>[2x]MPL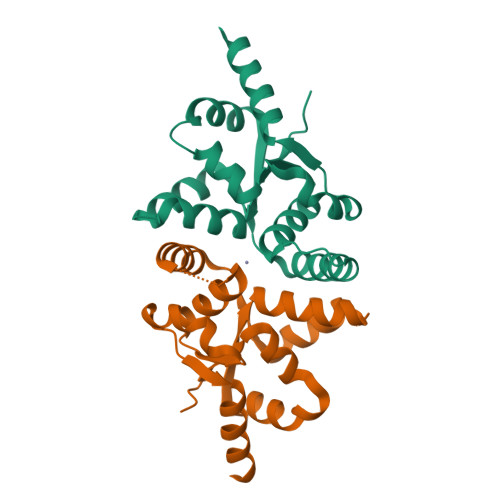PPDITFDSLALIKMHSQNMKRILEVTLAKFTVNLSIVTVYRYLTARAYLKKNIEAEFEILKDIYNIVPLLDDIAIKAAQIEANLIKKEITLDMEDIITATTAIYTNSLLVTDDPKRYEPIRRFGLDTMPLDKFIKEVELMVEKELI> NA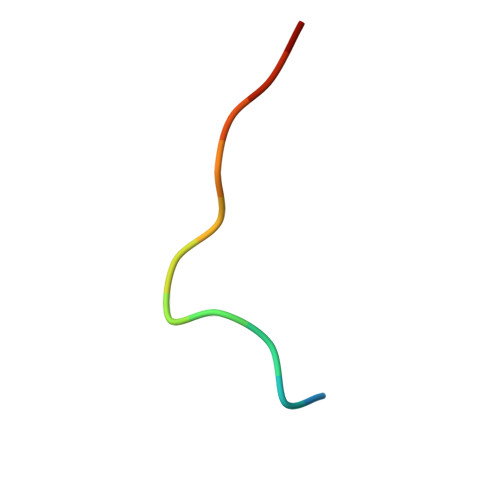FSPKYLLRLPQ> MDVFQEGLAMVVQDPLLCDLPIQVTLEEVNSQIALEYGQAMTVRVCKMDGEVMPVVVVQSATVLDLKKAIQRYVQLKQEREGGIQHISWSYVWRTYHLTSAGEKLTEDRKKLRDYGIRNRDEVSFIKKLRQK;> MNDWMPIAKEYDPLKAGSIDGTDEDPHDRAVWRAMLARYVPNKGVIGDPLLTLFVARLNLQTKEDKLKEVFSRYGDIRRLRLVRDLVTGFSKGYAFIEYKEERAVIKAYRDADGLVIDQHEIFVDYELERTLKGWIPRRLGGGLGGKKESGQLRFGGRDRPFRKPINLPVVKNDLYREGKRERRERSRSRERHWDSRTRDRDHDRGREKRWQEREPTRVWP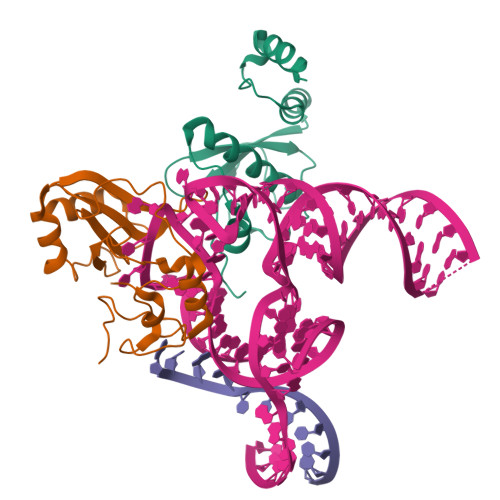DNDWERERDFRDDRIKGREKKERGK> MSTEHVDHKTIARFAEDKVNLPKVKADDFREQAKRLQNKLEGYLSDHPDFSLKRMIPSGSLAKGTALRSLNDIDVAVYISGSDAPQD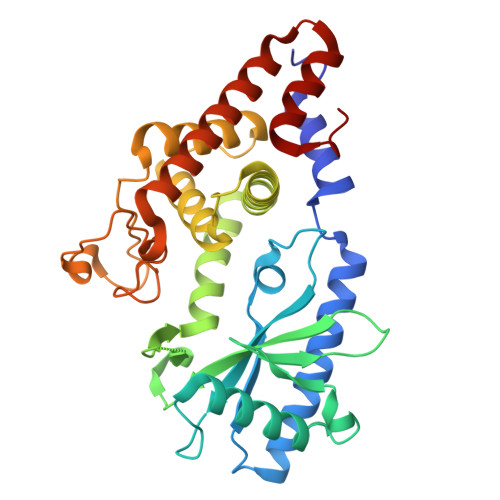LRGLLDYLADRLRKAFPNFSPDQVKPQTYSVTVSFRGSGLDVDIVPVLYSGLPDWRGHLISQEDGSFLETSIPLHLDFIKARKRAAPKHFAQVVRLAKYWARLMKQERPNFRFKSFMIELILAKLLDNGVDFSNYPEALQAFFSYLVSTELRERIVFEDNYPASKIGTLSDLVQIIDPVNPVNNVARLYTQSNVDAIIDAAMDAGDAIDAAFYAPTKQLTVTYWQKVFGSSFQG> TRKMWSVQESEWLKQGVVRYGVGHWERIRSAFPFAGRTAVNLKDRWRTMVKLKM;> TRKMWSVQESEWLKQGVVRYGV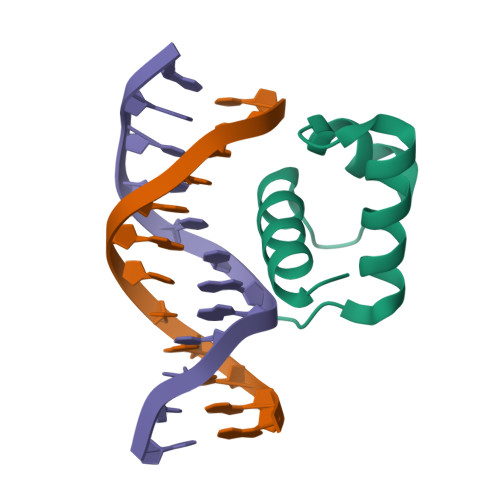GHWERIRSAFPFAGRTAVNLKDRWRTMVKLKMV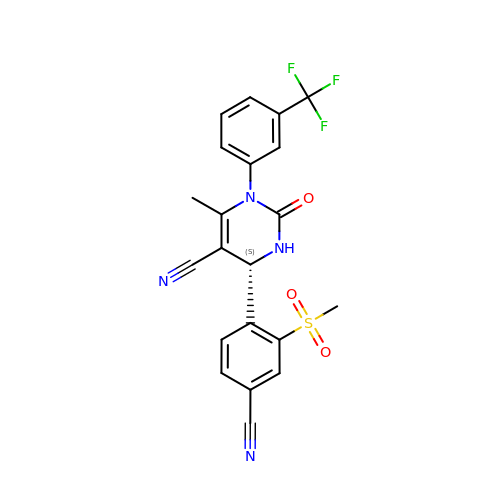(6S)-6-(4-cyano-2-methylsulfonyl-phenyl)-4-methyl-2-oxidanylidene-3-[3-(trifluoromethyl)phenyl]-1,6-dihydropyrimidine-5-carbonitrile | C21 H15 F3 N4 O3 S | WQASVWJQEKONLG-LJQANCHMSA-N> MSRLDKSKVINSALELLNEVGIEGLTTRKLAQKLGVEQPTLYWHVKN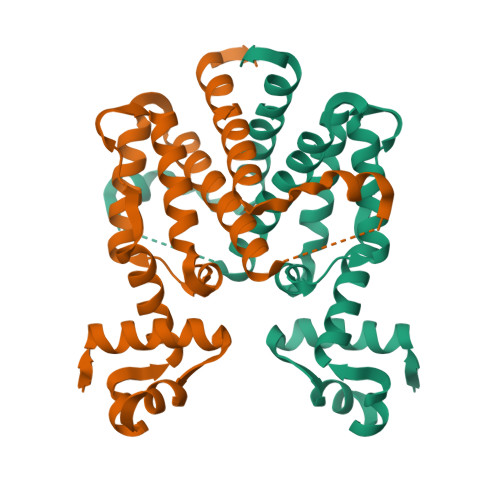KRALLDALAVEILARHHDYSLPAAGESWQSFLRNNAMSFRRALLRYRDGAKVHLGTRPDEKQYDTVETQLRFMTENGFSLRDGLYAISWVSHFTLGAVLEQQEHTAALTDRPAAPDENLPPLLREALQIMDSDDGEQAFLHGLESIIRGIEVQLTALLQIV;> GSHMSRLDKSKVINSALELLNEVGIEGLTTRKLAQKLGVEQPTLYWHVKNKRALLDALAVEILARHHDYSLPAAGESWQSFLRNNAMSFRRALLRYRDGAKVHLGTRPDEKQYDTVETQLRFMTENGFSLRDGLYAISAVSHATLGAVLEQQEHTAALTDRPAAPDENLPPLLREALQIMDSDDGEQAFLHGLEWLIRGFEVQLTALLQIV KDM6A (UTX) and KDM6B (JMJD3) are KDM6 subfamily members that catalyze demethylation of Nϵ-methylated histone 3 lysine 27 (H3K27), a mark important for transcriptional repression. Despite reports stating that UTY(KDM6C) is inactive as a KDM, we demonstrate by biochemical studies, employing MS and NMR, that UTY(KDM6C) is an active KDM. Crystallographic analyses reveal that the UTY(KDM6C) active site is highly conserved with those of KDM6B and KDM6A. UTY(KDM6C) catalyzes demethylation of H3K27 peptides in vitro, analogously to KDM6B and KDM6A, but with reduced activity, due to point substitutions involved in substrate binding.

Recently a small molecule inhibitor of KDM6A/B, GSK-J1, has been described. To ascertain whether UTY(KDM6C) showed an inhibitor profile similar to those of the other KDM6 subfamily members, a set of nine known KDM inhibitors were selected, and the response of KDM6A, UTY(KDM6C), and KDM6B to them (at 10 μm) was assessed, by measuring inhibition of demethylation of an H3K27Me3 peptide. All three KDMs displayed similar inhibition profiles, and, as anticipated, given its similarity to KDM6A, inhibition of UTY(KDM6C) activity by GSK-J1 was observed. GSK-J1 was the most potent inhibitor of KDM6B, KDM6A, and UTY(KDM6C) of the nine inhibitors tested. A structure of UTY(KDM6C) with GSK-J1 reveals that GSK-J1 is bound to the 2OG binding site identically within error to that observed with KDM6B·GSK-J1 complex; the propanoic acid of GSK-J1 is positioned to hydrogen-bond with Asn1103, Lys1084, and Thr1090, and the phenyl ring of the terahydrobenzazepine, as in the KDM6B·GSK-J1 complex, is sandwiched in a hydrophobic cleft between Arg948 and Pro1091. The pyridyl-pyrimidine biaryl heterocyclic GSK-J1 ring system is positioned to make bidentate interactions with the iron, and similarly to KDM6B, it translocates the iron ∼2.4 Å away from the HXE … H triad. Such metal movement has been observed with other 2OG oxygenases with certain iron-chelating inhibitors and may, in some circumstances, reflect potent inhibition. Further, crystal structures of the JmjC and Zn(II) domains of UTY(KDM6C) demonstrate that binding to both 2OG and the inhibitor, GSK-J1, displays identical structure to KDM6A/B. UTY(KDM6C) activity is also inhibited by small molecule probes developed as KDM6B inhibitors.

>MLPKDKLNPPTPSIYLENKRDAFFPPLHQFCTNPKNPVTVIRGLAGALKLDLGLFSTKTLVEANNEHMVEVRTQLLQPADENWDPTGTKKIWRCESNRSHTTIAKYAQYQASSFQESLREENEKRTQHKDHSDNESTSSENSGRRRKGPFKTIKFGTNIDLSDNKKWKLQLHELTKLPAFARVVSAGNLLTHVGHTILGMNTVQLYMKVPGSRTPGHQENNNFCSVNINIGPGDCEWFVVPEDYWGVLNDFCEKNNLNFLMSSWWPNLEDLYEANVPVYRFIQRPGDLVWINAGTVHWVQAVGWCNNIAWNVGPLTACQYKLAVERYEWNKLKSVKSPVPMVHLSWNMARNIKVSDPKLFEMIKYCLLKILKQYQTLREALVAAGKEVIWHGRTNDEPAHYCSICEVEVFNLLFVTNESNTQKTYIVHCHDCARKTSKSLENFVVLEQYKMEDLIQVYDQFTLALSLSSSSAENLYFQ[2x]> MADRIELRGLTVHGRHGVYDHERVAGQRFVIDVTVWIDLAEAANSDDLADTYDYVRLASRAA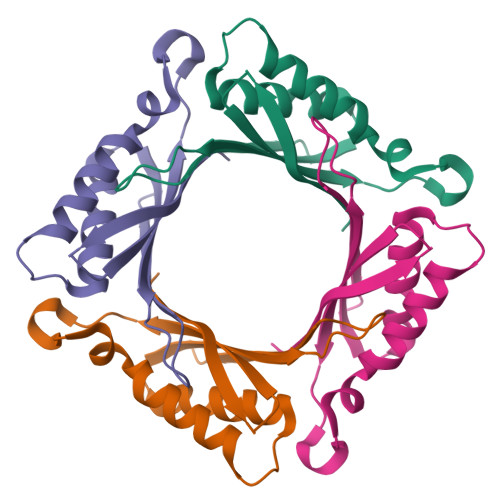EIVAGPPRKLIETVGAEIADHVMDDQRVHAVEVAVHKPQAPIPQTFDDVAVVIRRSRRGGRGWVVPAGGAV>[2x]GSNLGENKHYEVAKKCVEDLALYLKPLSGGKGVASLNQSALSRPMQRKLVTLVNCQLVEEEGRVRAMRAARSLGERTVTELILQHQNPQQLSANLWAAVRARGCQFLGPAMQEEALKLVLLALEDGSALSRKVLVLFVVQRLEPRFPQASKTSIGHVVQLL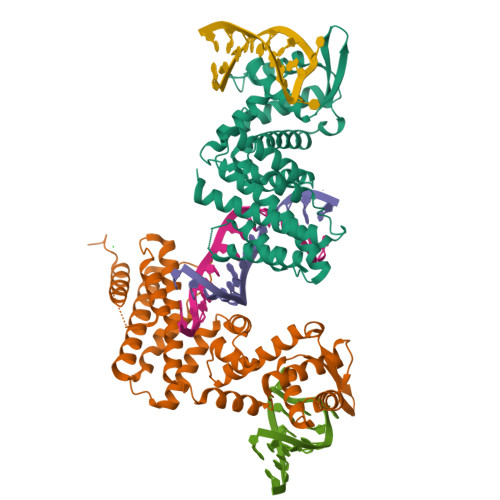YRASCFKVTKRDEDSSLMQLKEEFRSYEALRREHDAQIVHIAMEAGLRISPEQWSSLLYGDLAHKSHMQSIIDKLQSPESFAKSVQELTIVLQRTGDPANLNRLRPHLELLANIDPNPDAVSPTWEQLENAMVAVKTVVHGLVDFIQNYSRKGHETPQ> SFRTGE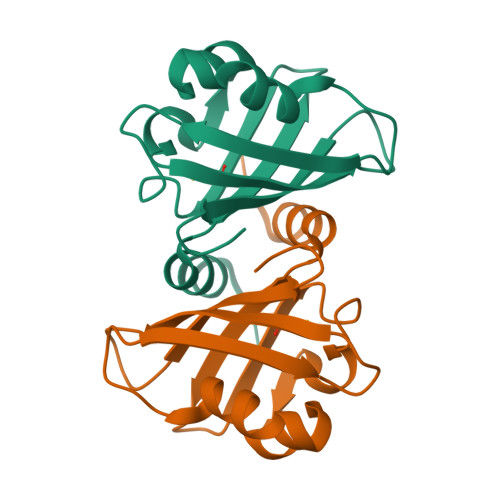RRIWDATATLEALGAADVALWIWEPETDRLRLNGAARALGLGPLAPECSSAAFRALALPQDRAQAEEVLKPREPGSEVVARFRVRGGETCLWRGVWLEEGVRAAGVVAPETKFSASELCDLTG N-(3-fluoropyridin-4-yl)-2-[6-(trifluoromethyl)pyridin-2-yl]-7H-pyrrolo[2,3-d]pyrimidin-4-amine 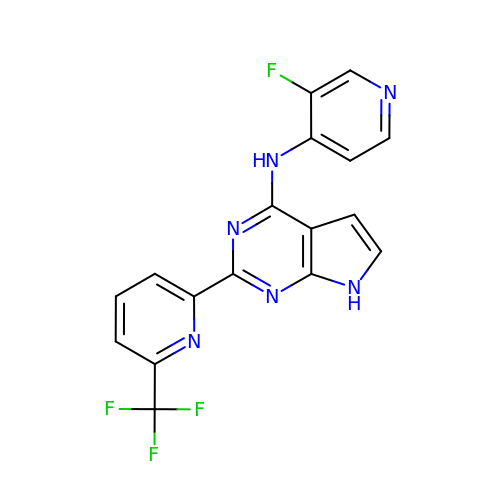| C17 H10 F4 N6 | KNTWBIUWHSYQJE-UHFFFAOYSA-N>GSEKPFKCSMCDYASVEVSKLKRHIRSHTGERPFQCSLCSYASRDTYKLKRHMRTHSGEKPYECYICHARFTQSGTMKMHILQKHTENVAKFHCPHCDTVIARKSDLGVHLRKQHSYIEQGKKCRYCDAVFHERYA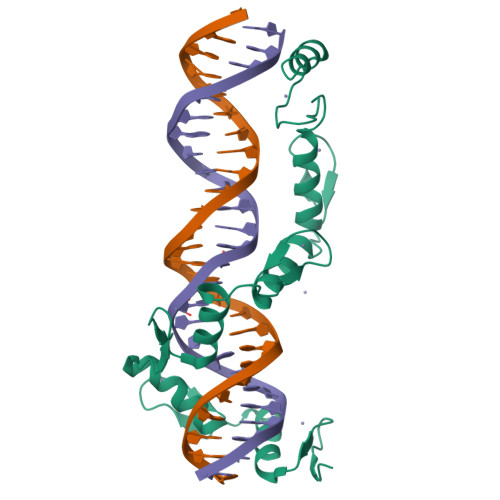LIQHQKSHKNEKRFKCDQCDYACRQERHMIMHKRTHTGEKPYACSHCDKTFRQKQLLDMHFKRYHD[2x]> GSSGIVMADWLKIRGTLKSWTKLWCVLKPGV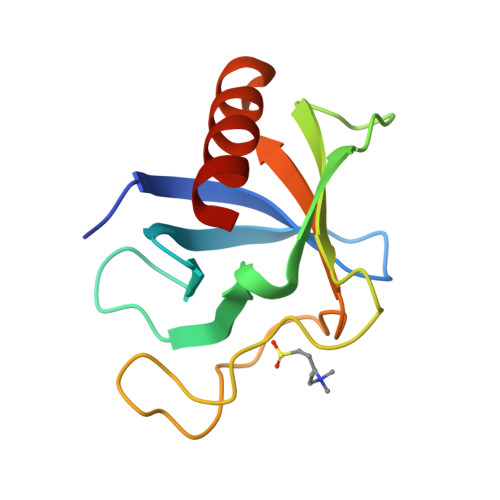LLIYKTQKNGQWVGTVLLNACEIIERPSKKDGFCFKLFHPLEQSIWAVKGPKGEAVGSITQPLPSSYLIIRATSESDGRCWMDALELALKSG> GAGCAGACAAG;> ACTGCACTCA;> CTAGT;> TCTGAGTGCTGTCTGC

In this work, we exhaustively probe the ability of all 36 immobile HJ sequences to form DNA crystals in two different designed systems. Three separate self-assembling DNA crystal systems are described in this report: the “4 × 5” and “4 × 6” designs (collectively referred to as the 4 × N systems), and a third construct with a “scrambled” sequence variant of the 4 × 6 lattices. Self-assembly was mediated by three constituent oligonucleotides: (S1) containing four sequence repeats of either 5 or 6 bases; (S2) composed of 21 bases containing complementary regions to both (S1); and (S3) which forms the second junction crossover. The HJ serves as the fundamental component at the core of each unit, and the ultimate assembly of the full lattice is facilitated by the complementary 2-base sticky ends that tail each duplex.

The 4 × 5 system robustly crystallized with 75% of the junctions, and we obtained crystals in all but 9 of 36 sequences. Of the resulting structures, 18 exhibited P32 symmetry with average cell dimensions a = b = 68.85 Å c = 60.09 Å, with only nine retaining the original P3221 symmetry with average cell edges a = b = 68.17 Å c = 60.60 Å. Although the cell parameters between the two symmetries were virtually indistinguishable, the differences between the periodicity of the lattices is dramatic, with vastly different cavity sizes. We hypothesize that even a small difference in junction angles could have a significant global effect on the assembly of the lattice, thereby eliminating the strain in the P3221 lattices. However, in the majority of the crystal structures reported here, the cacodylate anion indeed fits best into the electron density map of our X-ray structures, due to the presence of sodium cacodylate in the crystallization solution.Here, we explore the precise structural inhibitory mechanism of actinonin, which is a slow, tight-binding inhibitor of peptide deformylase (PDF), a metal cation-dependent enzyme. PDF is the first enzyme in the N-terminal methionine excision pathway, an essential and ubiquitous process that contributes to the diversity of N-terminal amino acids. The function of the active-site metal is to activate the reactive water molecule involved in peptide hydrolysis. Actinonin is a natural product with antibiotic activity that inhibits PDF by mimicking the structure of its natural substrates (nascent peptide chains starting with Fo-Met-Aaa, where Fo is a formyl group and Aaa is any amino acid) in their transition state.

In this respect, site-directed mutagenesis of AtPDF was performed on Gly41, Ile42, and Ile130. The two most interesting variants, G41Q and G41M, could be crystallized under the same conditions as the WT protein. In the case of G41Q, the structure of the apo-protein did not show any modifications compared to the WT structure and remained in an O conformation (“O” zone). The 3D structure of the variants in the absence of ligand is similar to that of WT, and a strict correlation exists between the completeness of the conformational change and both binding potency and catalytic efficiency.

> MEIVEYPDPILRAKNKRIDIFDENLKNLVDAMFDVMYKTDQIGLSAPQVGLNVQLMVFNPAGEPGEGKEIVLVNPKIKKYSDKLVPFDEGCLSFPGIYAEVVRPQSVKIDARDITGERFSISLSRLPARIFQHEYDHLEGVLFFDRMTDQVLDSIREELEALEKKYEEKTGLPSPERVEARQKRKAGVGFGKR>[2x]NLSQLSFHRVDQKEITQLSHLGQGTRTNVYEGRLRVEGSGDPEEGKMDDEDPLVPGRDRGQELRVVLKVLDPSHHDIALAFYETASLMSQVSHTHLAFVHGVCVRGPENIMVTEYVEHGPLDVWLRRERGHVPMAWKMVVAQQLASALSYLENKNL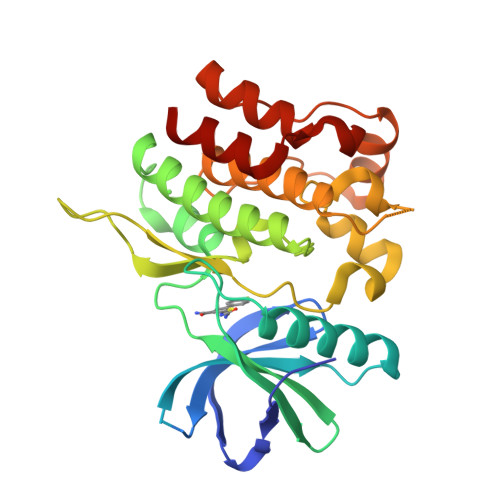VHGNVCGRNILLARLGLAEGTSPFIKLSDPGVGLGALSREERVERIPWLAPECLPGGANSLSTAMDKWGFGATLLEICFDGEAPLQSRSPSEKEHFYQRQHRLPEPSCPQLATLTSQCLTYEPTQRPSFRTILRDLTRL Orladeyo | C30 H26 F4 N6 O | 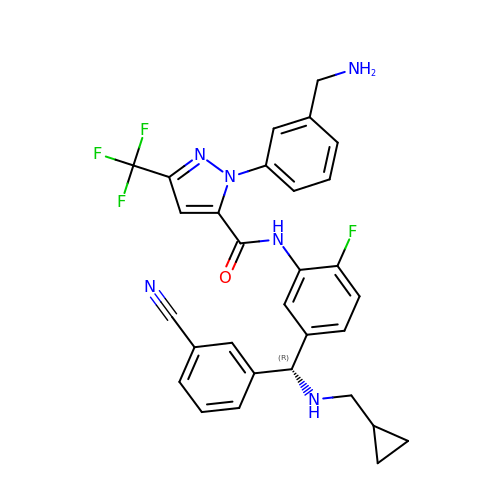UXNXMBYCBRBRFD-MUUNZHRXSA-N> GAHMGNWATHVYVPYEAKEEFLDLLDVLLPHAQTYVPRLVRMKVFHLSLSQSVVLRHHWI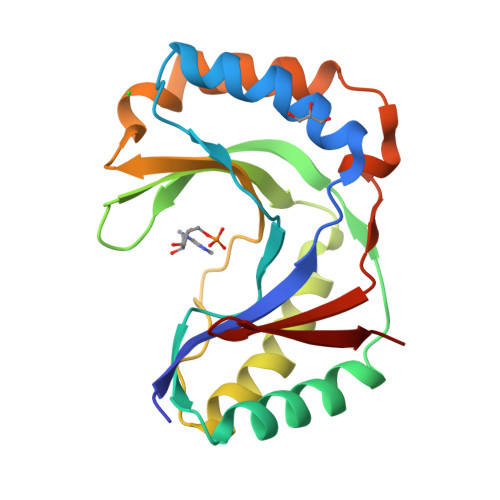LPFVQALKARMTSFHRFFFTANQVKIYTNQEKTRTFIGLEVTSGHAQFLDLVSEVDRVMEEFNLTTFYQDPSFHLSLAWCVGDARLQLEGQCLQELQAIVDGFEDAEVLLRVHTEQVRCKSGNKFFSMPLK> ISEFGSSHSTNDAKSPTLSESHKSARNVLENIGIKIYNQEIKKKNPYEQQLKGTLSRAQFVDALSSRYGYVRNSDGNSCNLDHLFHTNIKTGYNEGRKPCYGREQNRFDENAEAYCNSDKIRGNENNANGAACAPPRRRHICDQNLEFLDNKNTNTAHDLLGNVLVTAKYEGNYIVNDHPDKNSNGNKAGICTSLARSFADIGDIVRGRDMFLPNKDDKVQKGLQVVFKKIYKSLTPEARKHYAHGDGSGNYAKLREDWWTINREQIWKALTCSAPYYADYFRKGSDGTLHFSSHGKCGHNEGAPPTYLDYVPQFLRWFEEWSEEFCRIKKIKIDKVKKECRDEQNKKYCSGDGHDCTQTNLAHNQIFVDLDCPRCQDQCIKYNEWIVKKLEEFYKQNLKYSMEIQKWKKTKNNYYDKEFYENLDKKSYSTIDKFLNLLNNGKHCHDNKDEKNKIDFNKPIKTFSISEYCKTCPLYGVTCTNRGICIHNSNNKNKGENDLNKINIKDKSPTTFDVDMIYLRRQYMKNELKSFVESTCLFKGMRNQEWTCQILKNLDVCKLNNFNKVIDIDKHITFKVLLERWLKDFLEGYKKSKRKINPCTKDKNSCIKLCINKCTCVEEWLNKKEKEWGQIKKHFNKQFHGEGYDIAFKVKSYFEDNEADVRKSIDNFHVLKNKEEYEICNVDDNCRSQNNKKKKDIVTILLKELKDKIVSCKNQHKATKGKECCDKLPKIADGDTSDDEEQEDEAPAPPKPKPPSTPNPCVRKDQSGTHIVSVEDVAEWMQGVTHDRV

Rosetting, the capacity of infected red blood cells (RBCs) to bind uninfected RBCs, is a Plasmodium falciparum virulence factor. Rosetting is caused by a sub-group of PfEMP1 adhesins encoded by the large var gene family. The extracellular region of PfEMP1 comprises multiple adhesion domains called Duffy Binding-Like (DBL) and Cysteine-Rich Interdomain Region (CIDR). Nevertheless, the rosette-forming PfEMP1 adhesins described so far, namely IT4/R29, Palo Alto 89F5 VarO, 3D7/PF13_0003 and IT4/var60, belong to a specific sub-group called groupA/UpsA var genes and, interestingly, all four present a specific DBL1α1-CIDR1γ double domain Head region.

We determined the crystal structure of the double domain Head protein, the first structure of a multiple domain segment of PfEMP1, which reveals numerous interactions between the DBL1α1 and CIDRγ domains, and shows specific structural features of the CIDRγ class that differ from the published CIDRα class. The Head crystallised only in the presence of heparin, as found earlier for DBL1α1, with the best crystals diffracting to 2.8 Å resolution. The overall shape of the Head is rather compact, with the CIDR1γ domain folding back upon the DBL1α1 domain, thus burying a significant surface at the interface. The interface between the DBL1α1 and CIDR1γ domains is stabilised by several charged interactions (D367-D654, N381-R518, E389-Y521, Y437-K550) and, furthermore, a significant hydrophobic surface on DBL1α1 is buried within this interface. In CIDR1γ-VarO, this region (residues 496–570) contains a twisted antiparallel β-sheet composed of four strands (β1-4) as well as three short α-helices (H-2, 310H1, H-1), forming an N-terminal subdomain. All Cys residues are engaged in disulfide bridges except one free Cys (C604, canonical Cys(5) of CIDR1γ). Importantly, we clarified the structure of the NTS-DBL1α1 hinge region that was lacking in our previous structural analysis of the DBL1α1-VarO domain. We show that this region is surface-exposed and critical for RBC binding. Computer docking and site-directed mutagenesis localized a blood group A binding site in a restricted area situated at the interface of subdomain1 and subdomain 2 in the vicinity of the NTS-DBL1α1 hinge region. Importantly, the blood group A binding site and the major heparin-binding site that we mapped previously [37]are distant from each other on the surface, indeed on opposite sides of the molecule.>[3x]MLNLTKQMIEIRTILNKVDSSSAHLTLPSIVVIGSQSSGKSSVLESIVGREFLPKGSNMVTRRPIELTLVNTPNSNNVTADFPSMRLYNIKDFKEVKRMLMELNMAVPTSEAVSEEPIQLTIKSSRVPDLSLVDLPGYIQVEAADQPIELKTKIRDLCEKYLTAPNIILAISAADVDLANSSALKASKAADPKGLRTIGVITKLDLVDPEKARSILNNKKYPLSMGYVGVITKTPSSINRKHLGLFGEAPSSSLSGIFSKGQHGQSSGEENTNGLKQIVSHQFEKAYFKENKKYFTNCQVSTKKLREKLIKILEISMSNALEPTSTLIQQELDDTSYLFKVEFNDRHLTPKSYLLNNIDVLKLGIKEFQEKFHRNELKSILRAELDQKVLDVLATRYWKDDNLQDLSSSKLESDTDMLYWHKKLELASSGLTKMGIGRLSTMLTTNAILKELDNILESTQLKNHELI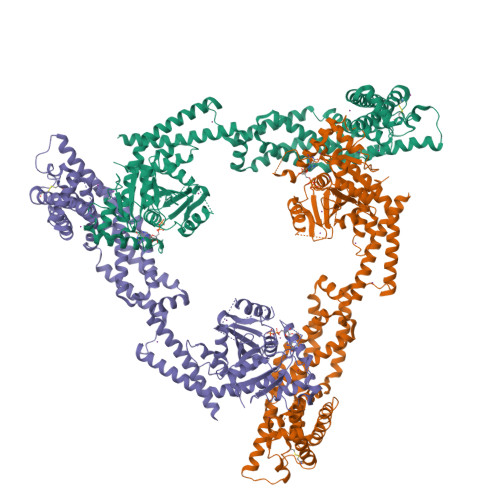KDLVSNTAINVLNSKYYSTADQVENCIKPFKYEIDLEERDWSLARQHSINLIKEELRQCNSRYQAIKNAVGSKKLANVMGYLENESNLQKETLGMSKLLLERGSEAIFLDKRCKVLSFRLKMLKNKCHSTIEKDRCPEVFLSAVSDKLTSTAVLFLNVELLSDFFYNFPIELDRRLTLLGDEQVEMFAKEDPKISRHIELQKRKELLELALEKIDSILVFKKSYKGVSKNL>[2x]SRVLLALHDRAPQLKISDDRLTVVGEKGYSMVRASHGVRKGAWYFEITVDEMPPDTAARLGWSQPLGNLQAPLGYDKFSYSWRSKKGTKFHQSIGKHYSSGYGQGDVLGFYINLPEDTISGRGSSEIIFYKNGVNQGVAYKDIFEGVYFPAISLYKSCTVSINFGPCFKYPPKDLTYRPMSDMG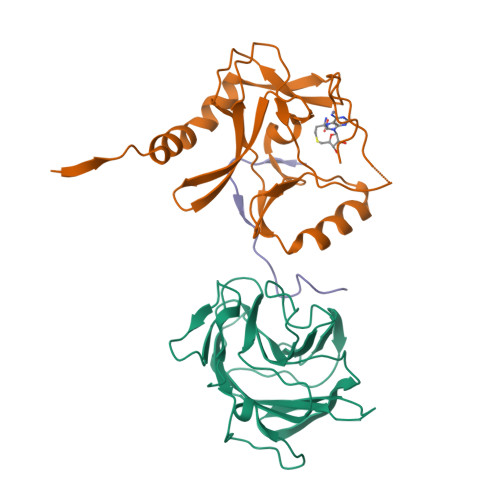;>STRRATSLELPMAMRFRHLKKTSKEAVGVYRSAIHGRGLFCKRNIDAGEMVIEYSGIVIRSVLTDKREKFYDGKGIGCYMFRMDDFDVVDATMHGNAARFINHSCEPNCFSRVIHVEGQKHIVIFALRRILRGEELTYDYKFPIEDASNKLPCNCGAKRCRRFLN[2x];>SAFAPDFKELDENVEYEERESEFDIED[2x]> MRIGIISVGPGNIMNLYRGVKRASENFEDVSIELVESPRNDLYDLLFIPGVGHFGEGMRRLRENDLIDFVRKHVED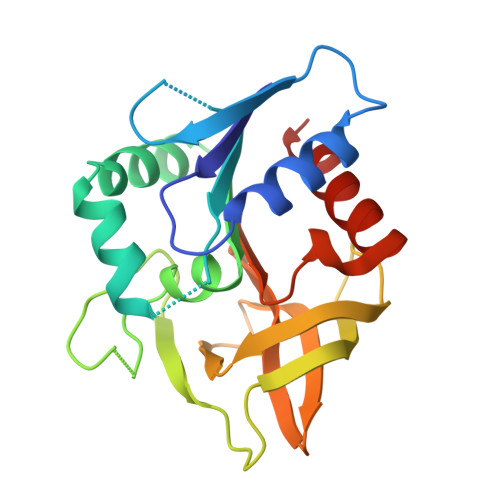ERYVVGVCLGMQLLFEESEEAPGVKGLSLIEGNVVKLRSRRLPHMGWNEVIFKDTFPNGYYAFVHTYRAVCEEEHVLGTTEYDGEIFPSAVRKGRILGFQFHPEASSKIGRKLLEKVIECSLSRR> DPPAVHLSNGPGQEPIAVMTFDLTKITKTSSSFEVRTWDPEGVIFYGDTNPKDDWFMLGLRDGRPEIQLHNHWAQLTVGAGPRLDDGRWHQVEVKMEGDSVLLEVDGEEVLRLRQVSGPLTSKRHPIMRIALGGLLFPASNLRLPLVP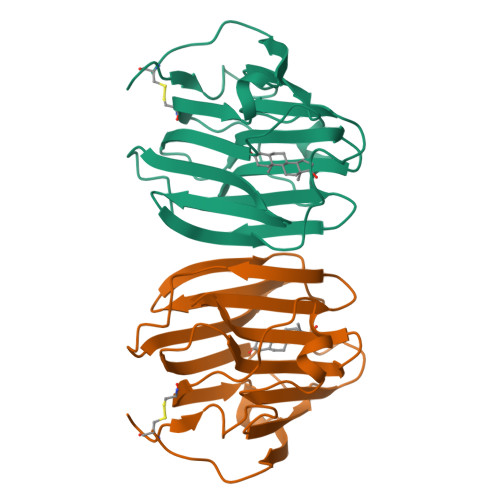ALDGCLRRDSWLDKQAEISASAPTSLRSC> MKKQNDIPQPIRGDKGATVKIPRNIERDRQNPDMLVPPETDHGTVSNMKFSFSDTHNRLEKGGYAREVTVRELPISENLASVNMRLKPGAIRELHWHKEAEWAYMIYGSARVTIVDEKGRSFIDDVGEGDLWYFPSGLPHSIQALEEGAEFLLVFDDGSFDSSNTFQLTDWLAHTPKEVIAANFGVTKEEISNLPGKEKYIFENQLPGSLKDDIVEGPNGEVPYPFTYRLLEQEPIESEGGKVYIADSTNFKVSKTIASALVTVEPGAMRELHWHPNTHEWQYYISGKARMTVFASDGHARTFNYQAGDVGYVPFAMGHYVENIGDEPLVFLEIFKDDHYADVSLNQWLAMLPETFVQAHLDLGK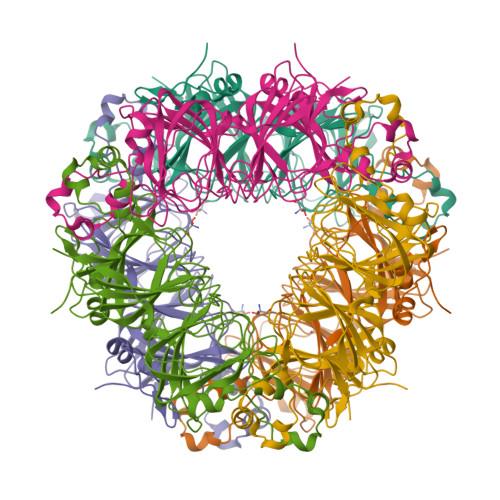DFTDVLSKEKHPVVKKKCSK> ANPYERGPDPTESSIEAVRGPFAVAQTTVSRLQADGFGGGTIYYPTDTSQGTFGAVAISPGFTAGQESIAWLGPRIASQGFVVITIDTITRLDQPDSRGRQLQAALDHLRTNSVVRNRIDPNRMAVMGHSMGGGGALSAAAQQTSLEAAIPLQGWHTRKQWSSVRTPTLVVGAELDTIAPVSSHSEAFYNSLPSDLDKAYMELRGASHTVSNTPDTTTAKYSIAWLKRFVDKDLRYEQFLCPAPDDFAISEYRSTCPFHHHHHH

Plastic pollution has become a global environmental challenge, driving interest in enzymatic polyethylene terephthalate (PET) recycling by using polyester hydrolases. Metagenome-derived polyester hydrolases, such as LCC and PHL7, have garnered significant attention due to their high activity at elevated temperatures of up to 70 °C. Their engineering led to the development of optimized variants, including LCCICCG, LCC-A2, Turbo-PETase, and PHL7mut3. , PHL7mut3 has been designed to improve the activity and thermostability of PHL7 by the Q175E, L210T, and D233 K mutations. In this study, the PHL7 wild-type enzyme and the improved PHL7 triple mutant PHL7mut3 were expressed in E. coli and P. pastoris, and their PET-degrading activity under various conditions as well as their thermal stability was assessed. Both the PHL7 and the PHL7mut3 sequences contain three putative N-glycosylation sites (N143, N144, and N161). To assess the impact of mutations and glycosylation on structural folding, we used X-ray crystallography to determine the structures of PHL7mut3, expressed in both E. coli (E_PHL7mut3) and P. pastoris (P_PHL7mut3), as well as a non-glycosylated variant with three additional mutations (P_PHL7mut3_ng), also expressed in P. pastoris.

To assess whether the enzymatic properties of the E. coli-produced enzymes can be reproduced when P. pastoris is used as a host, non-N-glycosylated enzyme variants were designed by substituting the asparagine (N) residues at the N-glycosylation sites with glutamine (Q) residues. Data for P_PHL7mut3_ng and P_PHL7mut3 were collected to resolutions of 1.02 and 1.37 Å, respectively. In the P_PHL7mut3 structure, electron density supported a single conformation for K233, whereas two conformations were modeled for the same residue in E_PHL7mut3 and P_PHL7mut3_ng. Very weak density indicates multiple conformations of K233 beyond the Cγ-atom in these two structures. We therefore consider the observed flexibility of K233 in the other two structures as characteristic for the enzyme in solution. The difference in the catalytic properties of E_PHL7mut3 and P_PHL7mut3_ng might be caused by the N143Q, N144Q, and N161Q mutations. Whereas N143 and N161 are highly solvent exposed, and mutation to a glutamine likely has little influence on PHL7 structure and dynamics; the N144Q mutation destroys the hydrogen-bonding interactions of the N144 side chain carboxamide group with Q104 and S146 because of steric hindrances. This difference might be primarily responsible for the observed catalytic differences between E_PHL7mut3 and P_PHL7mut3_ng. The mutations introduced to obtain non-glycosylated enzymes in P. pastoris resulted in a decrease in melting temperature compared to the E. coli-produced enzymes. In contrast, P_PHL7mut3_ng demonstrates a significantly lower initial slope, indicating a slower rate of PET degradation.> GLPTMNTPGSCQFLTSDDFQSPSAMPQYDVTPEMKIPGEVKNLMEIAEVDSVVPVQNVGEKVNSMEAYQIPVRSNEGSGTQVFGFPLQPGYSSVFSRTLLGEILNYYTHWSGSIKLTFMFCGSAMATGKFLLAYSPPGAGAPTKRVDAMLGTHVVWDVGLQSSCVLCIPWISQT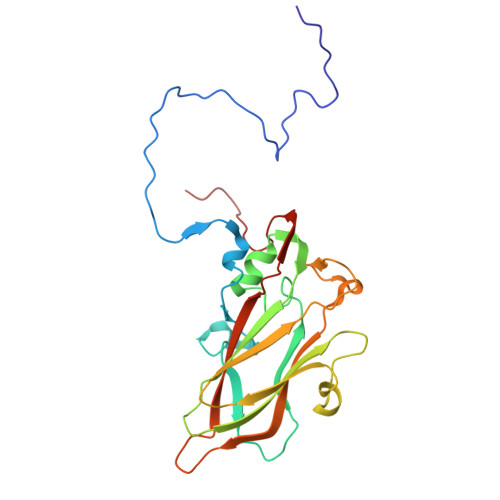HYRYVASDEYTAGGFITCWYQTNIVVPADAQSSCYIMCFVSACNDFSVRLLKDTPFISQNSFFQ> ADPEAFLLFSRRADIRRISLETNNNNVAIPLTGVKEASALDFDVTDNRIYWTDISLKTISRAFMNGSALEHVVEFGLDYPEGMAVDWLG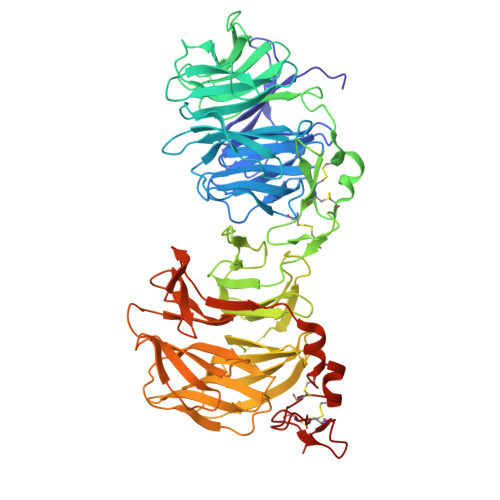KNLYWADTGTNRIEVSKLDGQHRQVLVWKDLDSPRALALDPAEGFMYWTEWGGKPKIDRAAMDGSERTTLVPNVGRANGLTIDYAKRRLYWTDLDTNLIESSNMLGLNREVIADDLPHPFGLTQYQDYIYWTDWSRRSIERANKTSGQNRTIIQGHLDYVMDILVFHSSRQSGWNECASSNGHCSHLCLAVPVGGFVCGCPAHYSLNADNRTCSAPTTFLLFSQKSAINRMVIDEQQSPDIILPIHSLRNVRAIDYDPLDKQLYWIDSRQNMIRKAQEDGSQGFTVVVSSVPSQNLEIQPYDLSIDIYSRYIYWTCEATNVINVTRLDGRSVGVVLKGEQDRPRAIVVNPEKGYMYFTNLQERSPKIERAALDGTEREVLFFSGLSKPIALALDSRLGKLFWADSDLRRIESSDLSGANRIVLEDSNILQPVGLTVFENWLYWIDKQQQMIEKIDMTGREGRTKVQARIAQLSDIHAVKELNLQEYRQHPCAQDNGGCSHICLVKGDGTTRCSCPMHLVLLQDELSCGEP>[2x]GHMPVRYFIMKSSNLRNLEISQQKGIWSTT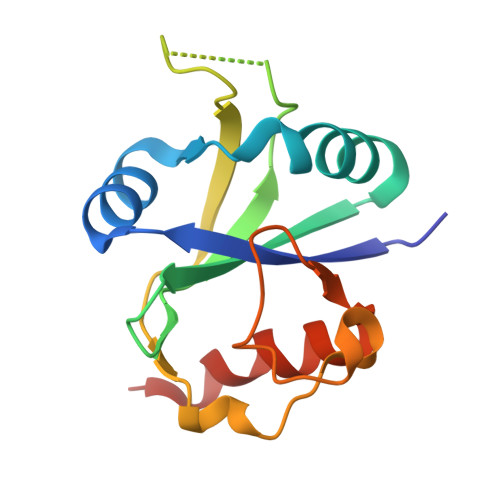PSNERKLNRAFWESSIVYLVFSVQGSGHFQGFSRMSSEIGREKSQDWGSAGLGGVFKVEWIRKESLPFQFAHHLLNPWNDNKKVQISRDGQELEPLVGEQLLQLWERLPLGEK>SNAMEIICFGDSITRGYDVPYGRGWVEICDASIENVNFTNYGEDGCSVQGMIYNIENWAVTAVSDPTRHIFLMCGTNDILQGRDSTYVYKTLVKAIELASTKGMVIIGLETQIDSDMDGLDLVVREVNEQLKAYAAEHNIKVIDFYTTLFEADQIGQIVFAGE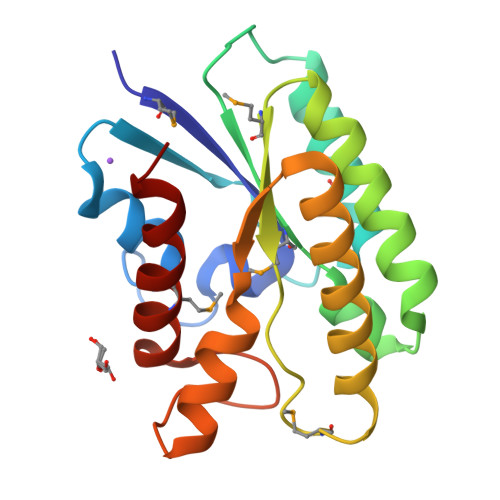VHPNERGYRLMAYKALEVFTRL[2x]>APTGDPACRAAVATAQKIAPLAHGEVAALTMASAPLKLPDLAFEDADGKPKKLSDFRGKTLLVNLWATWCVPSRKEMPALDELQGKLSGPNFEVVAINIDTRDPEKPKTFLKEANLTRLGYFNDQKAKVFQDLKAIGRALGMPTSVLVDPQGCEIATIAGPAEWASEDALKLIRAATGKAAAAL[4x];>W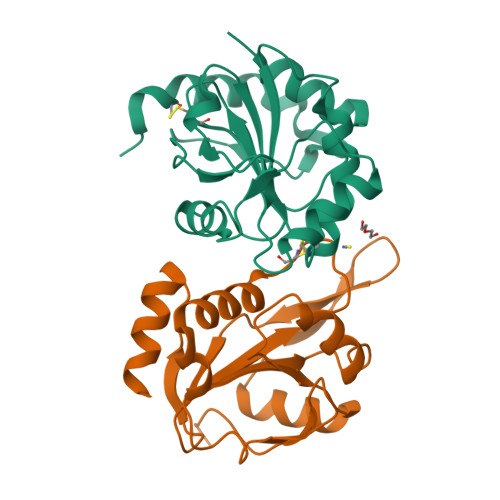SHPQFEKGGVGKVAQPAAIGGPFQLTDQNGKAVTDKSLKGKPTLIFFGYTHSPDVCPTSLFEISEVLRAMGKDADKVNAIFISVDPERDTPATMKNYLSSFDPHLEGLSGDPAEIAKVITSYRVYAKKVPTKDGDYTMDHTALIYLMDRDGRFVSPFNLKRTPEEAAADLKRYL[4x]cyclobutanecarboxylic acid | C5 H8 O2 | 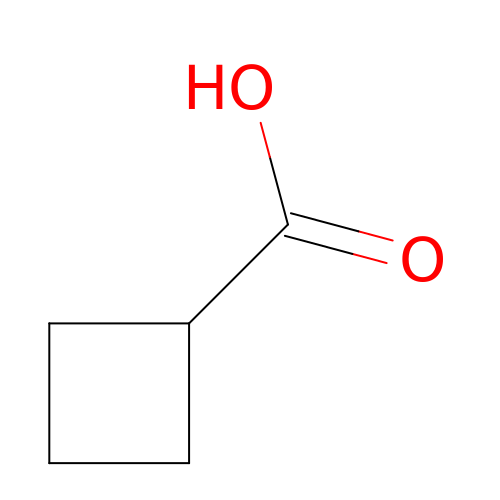TXWOGHSRPAYOML-UHFFFAOYSA-N OCTAN-1-OL | C8 H18 O | 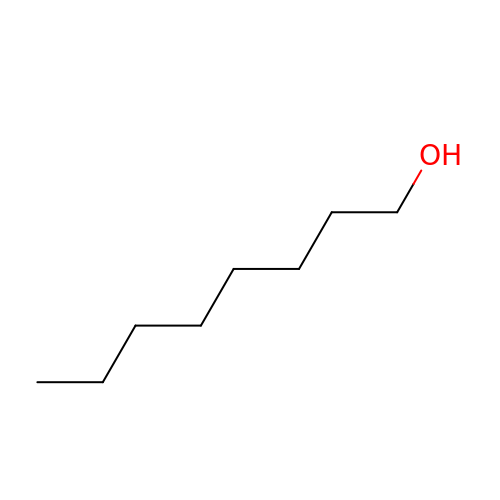KBPLFHHGFOOTCA-UHFFFAOYSA-N> APAPVKQGPTSVAYVEVNNNSMLNVGKYTLADGGGNAFDVAVIFAANINYDTGTKTAYLHFNENVQRVLDNAVTQIRPLQQQGIKVLLSVLGNHQGAGFAN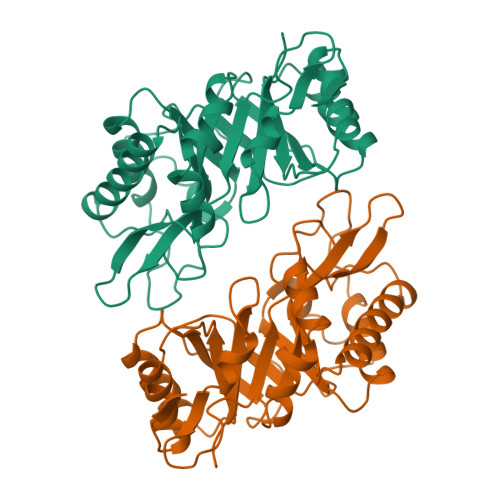FPSQQAASAFAKQLSDAVAKYGLDGVDFDDEYAEYGNNGTAQPNDSSFVHLVTALRANMPDKIISLYNIGPAASRLSYGGVDVSDKFDYAWNPYYGTWQVPGIALPKAQLSPAAVEIGRTSRSTVADLARRTVDEGYGVYLTYNLDGGDRTADVSAFTRELYGSEAVRTP PYRIDINE-2,4-DICARBOXYLIC 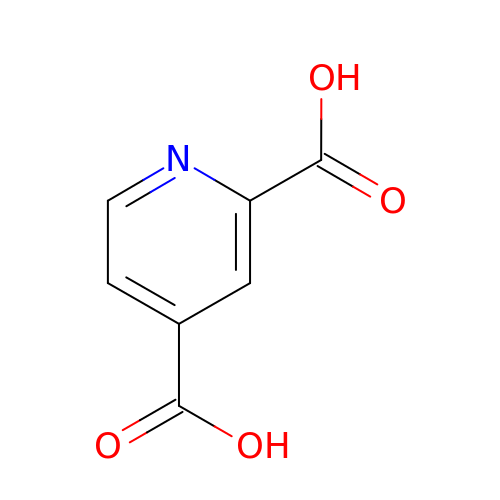ACID | C7 H5 N O4 | MJIVRKPEXXHNJT-UHFFFAOYSA-N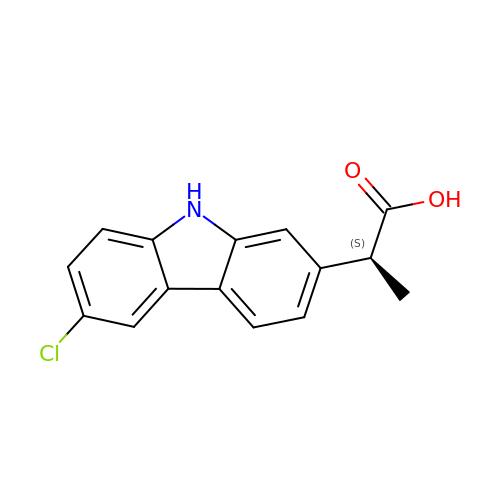(2S)-2-(6-chloro-9H-carbazol-2-yl)propanoic acid | C15 H12 Cl N O2 | PUXBGTOOZJQSKH-QMMMGPOBSA-N>[3x]MIHLYDAKSFAKLRAAQYAAFHTDAPGSW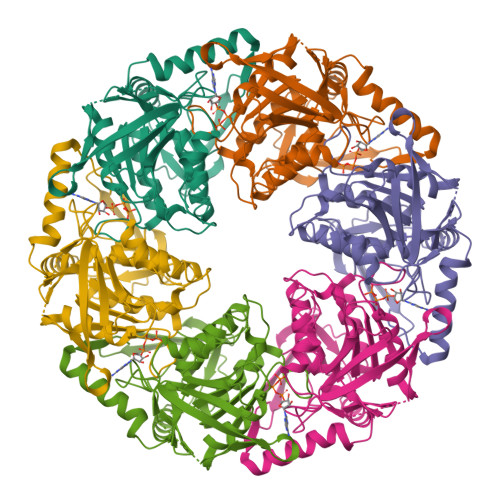FDHTSGVLESVEDGTPVLAIGVESGDAIVFDKNAQRIVAYKEKSVKAEDGSVSVVQVENGFMKQGHRGWLVDLTGELVGCSPVVAEFGGHRYASGMVIVTGKGNSGKTPLVHALGEALGGKDKYATVRFGEPLSGYNTDFNVFVDDIARAMLQHRVIVIDSLKNVIGAAGGNTTSGGISRGAFDLLSDIGAMAASRGCVVIASLNPTSNDDKIVELVKEASRSNSTSLVISTDVDGEWQVLTRTGEGLQALTHTLQTSYGEHSVLTIHTSKQSGGKQASGKAIQTVIKNDELESVLRRLTSN>VIDPSELTFVQEIGSGQFGLVHLGYWLNKDKVAIKTIREGAMS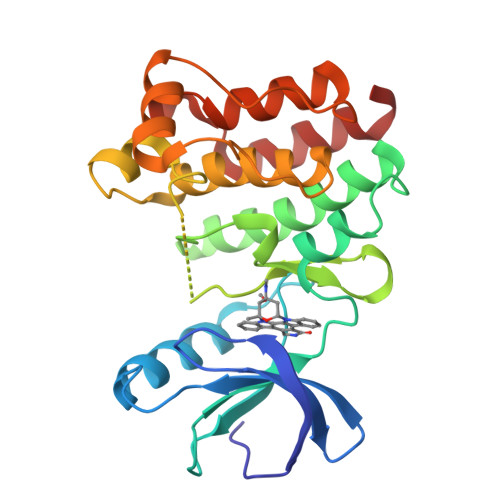EEDFIEEAEVMMKLSHPKLVQLYGVCLEQAPICLVFEFMEHGCLSDYLRTQRGLFAAETLLGMCLDVCEGMAYLEEACVIHRDLAARNCLVGENQVIKVSDFGMTRFVLDDQYTSSTGTKFPVKWASPEVFSFSRYSSKSDVWSFGVLMWEVFSEGKIPYENRSNSEVVEDISTGFRLYKPRLASTHVYQIMNHCWKERPEDRPAFSRLLRQLAEIAESGL[2x]> MSTSTEKRSKENLPWVEKYRPETLDEVYGQNEVITTVRKFVDEGKLPHLLFYGPPGTGKTSTIVALAREIYGKNYSNMVLELNASDDRGIDVVRNQIKDFASTRQIFSKGFKLIILDEADAMTNAAQNALRRVIERYTKNTRFCVLANYAHKLTPALLSRCTRFRFQPLPQEAIERRIANV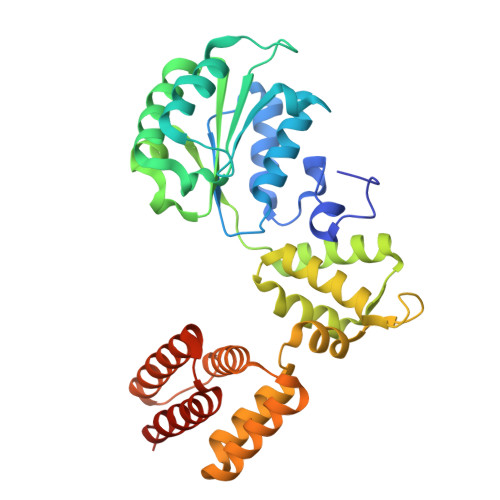LVHEKLKLSPNAEKALIELSNGDMRRVLNVLQSCKATLDNPDEDEISDDVIYECCGAPRPSDLKAVLKSILEDDWGTAHYTLNKVRSAKGLALIDLIEGIVKILEDYELQNEETRVHLLTKLADIEYSISKGGNDQIQGSAVIGAIKASFENETVKANV> CCGGGCC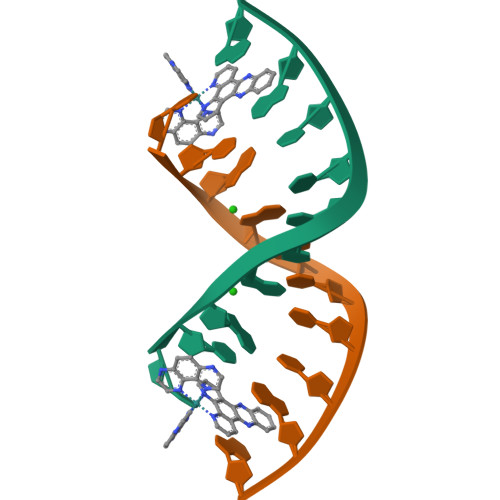CGG> SNASKELKVLVLCAGSGTSAQLANAINEGANLTEVRVIANSGAYGAHYDIMGVYDLIILAPQVRSYYREMKVDAERLGIQIVA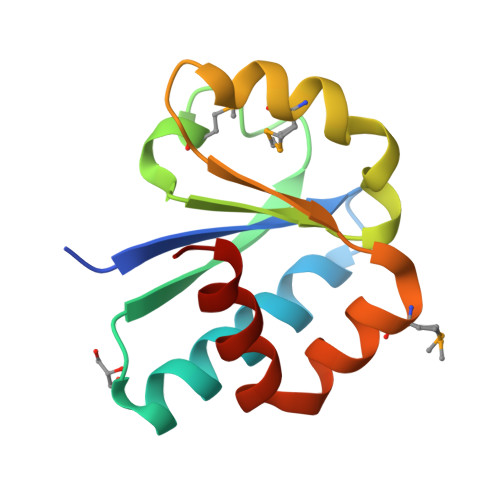TRGMEYIHLTKSPSKALQFVLEHYQ For rotaviruses (RVs), which are the major causative agents of life-threatening gastroenteritis in children under the age of 5 years and result in 453,000 deaths worldwide annually, recognition of specific cellular glycans for initial cell attachment is mediated by the distally located VP8* domain of the spike protein VP4. Although structurally conserved with a galectin-like fold, sequence-wise VP8* is the least conserved among RV structural proteins contributing to a phylogeny consisting of 37 [P] genotypes9. Our crystallographic analyses provide the structural basis to explain the unique glycan specificity exhibited by a neonate-specific bovine-human reassortant RV strain and its parental bovine strain, each belonging to the P genotype. We have shown that P VP8* exhibits a novel glycan-binding site that adapts to a differential recognition of precursor glycans, which are the core elements of HBGA and human/bovine milk glycans.

To investigate how P HRV VP8* can also bind to Galβ-GlcNAc motif with β1,3 linkage, we determined the structure of P HRV VP8* in complex with LNT to a resolution of 1.5 Å. The residues N155, Y156, W178, G179 and D185, which provide hydrophobic interactions with the terminal Galβ1,4-GlcNAc moieties of LNnT, now interact with the reducing end Galβ1,4-Glc of LNT sharing a common set of hydrogen bond and hydrophobic interactions. The non-reducing terminal Galβ1,3-GlcNAc of LNT, because of the shift, makes a new set of hydrophobic interactions involving I158, S180 and Y183. Comparison of the unliganded and LNT-bound P VP8* structures also showed that ligand binding induces significant changes. The R154 side chain that pairs with the aromatic side chain of F143 via a cation–π interaction in the unliganded structure, upon LNT binding, swings around to interact with the Gal3 residue, through a water-mediated hydrogen bond, and the side chain of F143 rotates accordingly to maintain the cation–π interaction. The side chain of S180 that hydrogen bonds with the main chain NH of Y183 in the unliganded structure reorients upon LNT binding to interact with the GlcNAc moiety through a water-mediated hydrogen bond interaction. A significant change that is observed in the LNT-bound structure is with respect to Y183 in the J-K loop. The side chain of Y183 is rotated to create a hydrophobic pocket to stabilize the terminal Galβ1,3-GlcNAc of LNT. Without this side chain reorientation, Y183 would clash with the GlcNAc residue.

> GSALDGPYTPDSSNLPSNYWYLINPLNDGVVFSVTNNSTFWMFTYLILPNTAQTNVTVNVMNETVNISIDNSGSTYRFVDYFKTSSTQSYRQRNYLITEHRLQAYRRDESGNISNYWGSSTYGDLRVGTYFNPVLNAVINLNADFYIIPDSQQEKCTEYIKGGL>MELESIQCDLSAFPGVKFFRIEAIFRPWRLPFVIDTLSKYGIRGLTNTPVKGVGVQGGSRERYAGTEFGPSNLVDKEKLDIVVSRAQVDAVVRLVAASAYTGEIGDGKIFVHPVAEVVRIRTAETGLEAEKMEGGMEDMMKKKK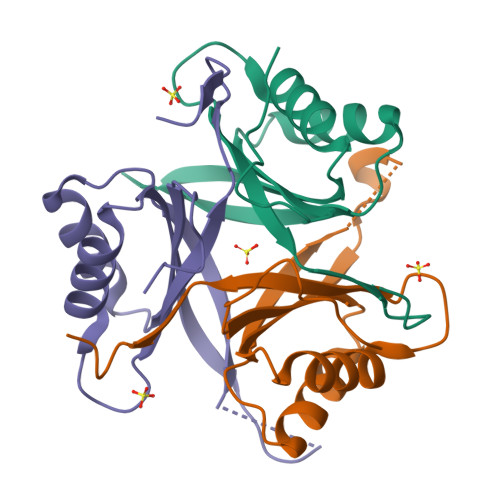SAWSHPQFEK[3x]Thus, the ZrgA proteins appear to represent a newly discovered family of zinc SBPs widespread among Gram-negative bacteria, including human pathogens. Here, we have determined the crystal structure of ZrgA from Vibrio cholerae and characterized its zinc binding in vitro and function in vivo. ZrgA adopts a ferredoxin-like fold, albeit with different topology from the classic ferredoxin (fd), that bears no similarity to known SBPs. Here, we show that ZrgA likely functions as the SBP for the ZrgBC permease/ATPase transporter system as it is required for normal growth and survival in zinc-deficient conditions in the ΔznuA background.

Since zinc-bound ZrgA would not crystallize, zinc was soaked into crystals of apo Δ124-184 ZrgA to acquire the holo protein structure at 2.41 Å resolution. We also acquired a dataset at the zinc absorption edge to generate an anomalous density map, which allowed us to model a total of 21 zinc ions into the asymmetric unit. These fall into 5 different binding sites. Sites 1 and 2 are observed in every chain with strong anomalous density and relatively low B-factors for the zinc ion. Site 1 is coordinated by the previously disordered His 35 and His 37 as well as Glu 66. Site 1 is conserved in PA4063 where a fourth His aligning with His 184 in ZrgA coordinates the metal. Site 2 is observed on the long alpha helix and is shared between two chains, one containing ligands Glu 83, His 86 and His 87, the other contributing Glu 79. Site 3 is located at the opposite end of the protein from site 1 and is coordinated by residues His 49, His 194, and Glu 196. Although the structures of apo and holo ZrgA are very similar with RMSD ~ 0.5 Å, they do reveal a few interesting conformational changes accompanying zinc binding, particularly near site 1. Further, the loop containing Glu 66 moves approximately 4 Å to allow zinc coordination.

>DHHSDHQHRQHEAHVHGQVELNIAQDGHDLLLEITAPGADVVGFEHAPQDDAQKQALEKALETLHHPEKLFALSDKAQCEKREVLIKHTLGGEEYQHSHAYGGSFTAQYQFHCEAVDQLKQIDTQWFQYFPSTEKIQANVLTEKQQSALQLNAKQTLIKL[6x]> RTFSYTLEDHTKQAFGIMNELRLSQQLCDVTLQVKYQDAPAAQFMAHKVVLASSSPVFKAMFTNGLREQGMEVVSIEGIHPKVMERLIEFAYTASISMGEKCVLHVMNGAVMYQIDSVVRACADFLVQQLD

A major step forward was the discovery in 1999 that the primary repressor of NRF2 is KEAP1, with 27 cysteines in humans, 25 of which are highly conserved. To determine the pKa of KEAP1 C151, we used a construct containing only three cysteines (versus 27 in full-length KEAP1) consisting of just the BTB (Broad-Complex, Tramtrack and Bric-a-brac) domain (residues 48–180, with a S172A mutation), which has been widely employed for crystallographic studies of C151-targeted electrophiles.

To assess the protonation state of C151 at various pHs, the thiolate-reactive probe monobromobimane (mBBr) was used, as it produces a fluorescent monobimane-thiol conjugate. In contrast, for the C151S BTB protein, the protein was unmodified by monobimane, confirming that only C151 is modified in WT BTB. Positive electron density near C151 indicated that ligand was bound. However, the density was ambiguous and not continuous, suggesting that the ligand was flexibly bound and adopting multiple conformations. C151-conjugated monobimane was also docked using this method. The scores overall were lower than for the pre-covalent docking, and again, no one pose had a distinctly larger and more negative docking score than the others, supporting our hypothesis that the lack of clear electron density for monobimane in the crystal structure is the result of the ligand adopting multiple conformations. Overall, the data suggest that monobromobimane, with its relatively flat geometry, largely hydrophobic nature, and possibly its ability to make hydrogen bonds, fits well into the relatively flat, hydrophobic C151 pocket in multiple orientations that place its electrophilic carbon near the C151 thiolate, significantly accelerating the reaction relative to the simple thiolate in NAC.>MKPVLL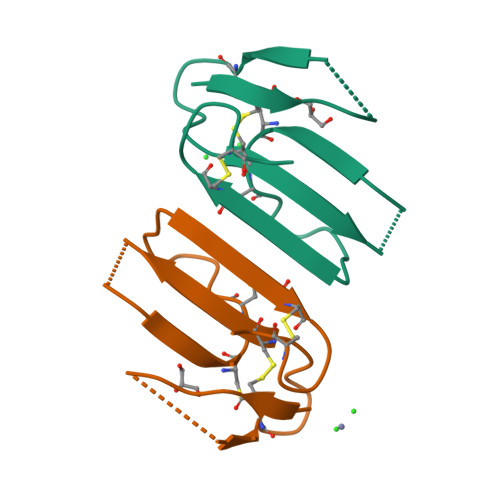TLVVVTIVCLDLGYTRICLKQEPFQPETTTTCPEGEDACYNLFWSDHSEIKIEMGCGCPKTEPYTNLYCCKIDSCNK[2x]> QSKET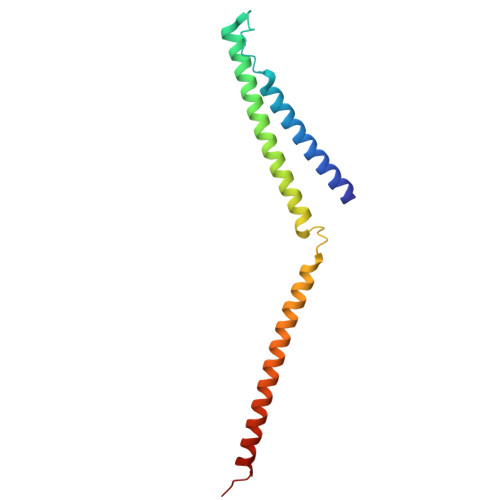LLQSYNKRLKDDIKSIMDNFTEIIKTAKIEDETQVSRATQGEQDNYEMHVRAANIVRAGESLMKLVSDLKQFLILNDFPSVNEAIDQRNQQLRALQEECDRKLITLRDEVSIDLYELEEEYYSSSS>[2x]MEEMPLRESSPQRAERCKKSWL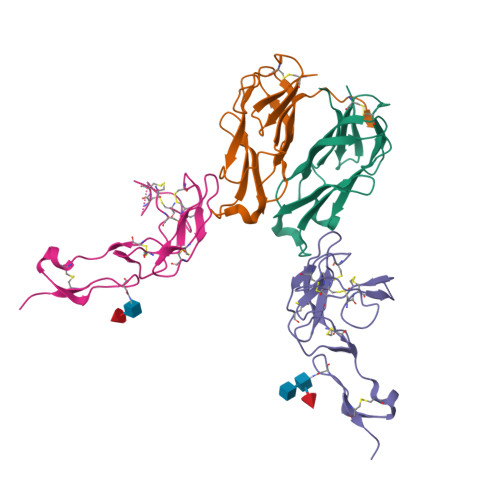LCIVALLLMLLCSLGTLIYTSLKPTAIESCMVKFELSSSKWHMTSPKPHCVNTTSDGKLKILQSGTYLIYGQVIPVDKKYIKDNAPFVVQIYKKNDVLQTLMNDFQILPIGGVYELHAGDNIYLKFNSKDHIQKTNTYWGIILMPDLPFIS;>[2x]MGAWAMLYGVSMLCVLDLGQPSVVEEPGCGPGKVQNGSGNNTRCCSLYAPGKEDCPKERCICVTPEYHCGDPQCKICKHYPCQPGQRVESQGDIVFGFRCVACAMGTFSAGRDGHCRLWTNCSQFGFLTMFPGNKTHNAVCIPEPLPTEQYGHLTVIFLVMAACIFFLTTVQLGLHIWQLRRQHMCPRETQPFAEVQLSAEDACSFQFPEEERGEQTEEKCHLGGRWP> NQVLVPNLNPTPENLEVVGDGFKITSSINLVGEEEADENAVNALREFLTANNIEINSENDPNSTTLIIGEVDDDIPELDEALNGTTAENLKEEGYALVSNDGKIAIEGK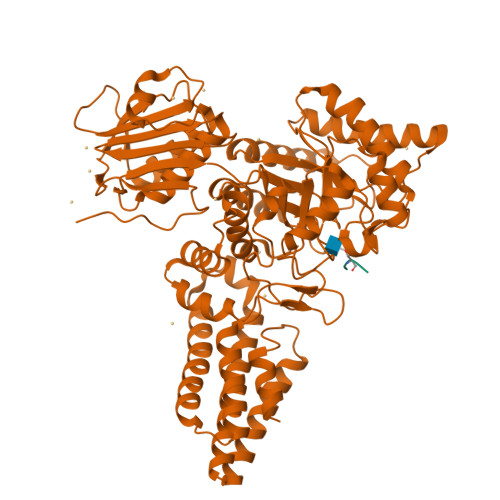DGDGTFYGVQTFKQLVKESNIPEVNITDYPTVSARGIVEGFYGTPWTHQDRLDQIKFYGENKLNTYIYAPKDDPYHREKWREPYPESEMQRMQELINASAENKVDFVFGISPGIDIRFDGDAGEEDFNHLITKAESLYDMGVRSFAIYWDNIQDKSAAKHAQVLNRFNEEFVKAKGDVKPLITVPTEYDTGAMVSNGQPRAYTRIFAETVDPSIEVMWTGPGVVTNEIPLSDAQLISGIYDRNMAVWWNYPVTDYFKGKLALGPMHGLDKGLNQYVDFFTVNPMEHAELSKISIHTAADYSWNMDNYDYDKAWNRAIDMLYGDLAEDMKVFANHSTRMDNKTWAKSGREDAPELRAKMDELWNKLSSKEDASALIEELYGEFARMEEACNNLKANLPEVALEECSRQLDELITLAQGDKASLDMIVAQLNEDTEAYESAKEIAQNKLNTALSSFAVISEKVAQSFIQEAL;> PSTA> KKQTQRNVFRCNVIGVKNCGKSGVLQALLGRNLMRQKKIREDHKSY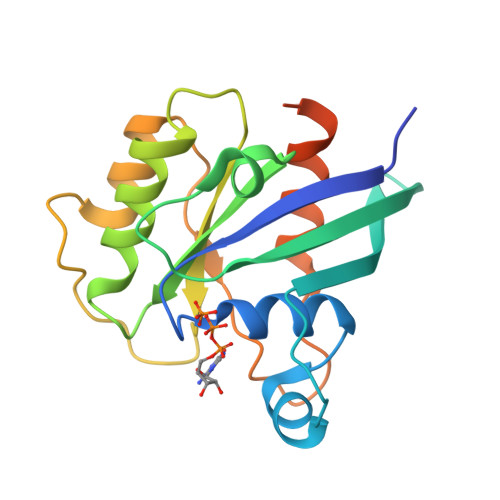YAINTVYVYGQEKYLLLHDISESEFLTEAEIICDVVCLVYDVSNPKSFEYCARIFKQHFMDSRIPCLIVAAKSDLHEVKQEYSISPTDFCRKHKMPPPQAFTCNTADAPSKDIFVKLTTMAMYPHVTQADLKSSTFLEHHHHHH>[8x]MGSSHHHHHHSSGRENLYFQGHMYV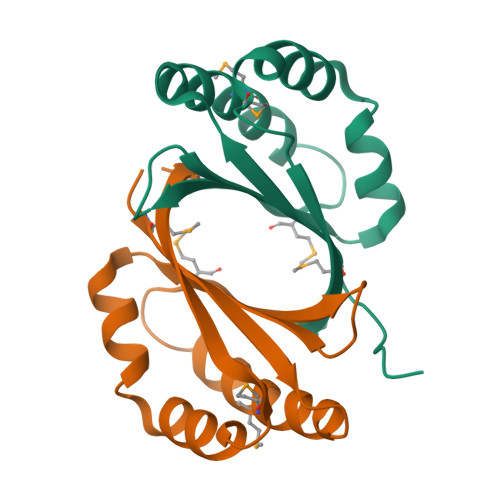TIVYASVKTDKTEAFKEATRMNHEQSIREPGNMRFDILQSADDPTRFVLYEAYKTRKDAAAHKETAHYLTWRDTVADWMAEPRKGVIYGGLYPTGDDGS> MKKIEAIIRPFKLDEVKIALVN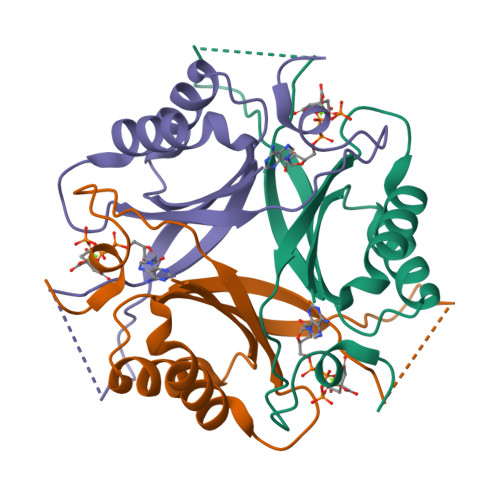AGIVGMTVSEVRGFGRQKGQTERYRGSEYTVEFLQKLKLEIVVEDAQVDTVIDKIVAAARTGENGDGKIFVSPVDQTIRIRTGEKNADAISAWS>[2x]ASGLVASNLNLKPGECLRVRGEVAPDAKSFVLNLGKDSNNLCLHFNPRFNAHGDANTIVCNSKDDGAWGTEQREAVF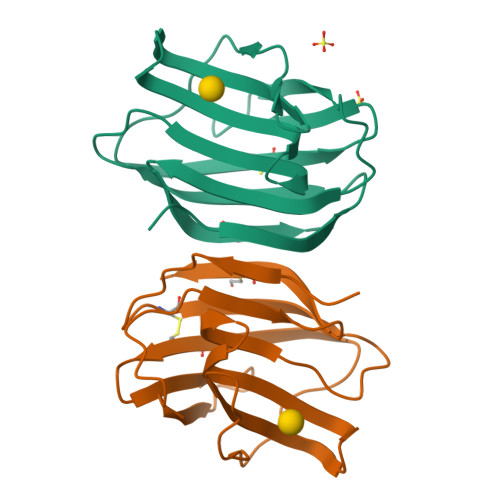PFQPGSVAEVCITFDQANLTVKLPDGYEFKFPNRLNLEAINYMAADGDFKIKCVAFD>[2x]MELQPQFNEFLANIRPTDTQKEDWKSGARTLRERLKNFEPLKEIVVSTFLQGSIRRSTAIRPLGDKRPDVDIVVVTNLDHTRMSPTDAMDLFIPFLEKYYPGKWETQGRSFGITLSYVELDLVITAIPESGAEKSHLEQLYKSESVLTVNSLEEQTDWRLNKSWTPNTGWLSESNSAQVEDAPASEWKAHPLVLPDREKNEWGRTHPLAQIRWTAEKNRLCNGHYINLVRAVKWWR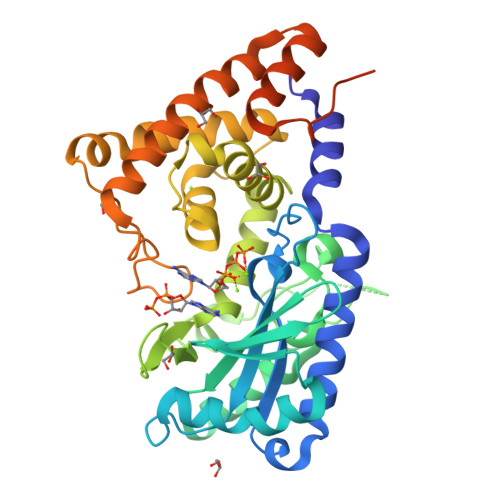QQNSEDLPKYPKGYPLEHLIGNALDNGTTSMAQGLVQLMDTFLSRWAAIYNQKSKPWLSDHGVAEHDVMARLTAEDFCSFYEGIASAAEIARNALASEEPQESAQLWRQLFGSKFPLPGPQGGDRNGGFTTPSKPAEPQKTGRFALEHHHHHH>MNVSIEEFTHFDFQLVPEPSPLDLVITESLKNHIEVNGVKSGALLPLPFQTGIGKTYTALNFLLQQMLEQVRSELKEENTGKKSKRLLYYVTDSVDNVVSAKADLLKLIEKQTVKGEPRFTLEQQEYLKAQIVHLPNQSEQLLQCSDAVLNDVLIGFNLNAERDVQAEWSAISGLRRHASNPEVKISLNRQAGYFYRNLIDRLQKKQKGADRVLLSGSLLASVETLLPGEKIRNGSAHVAFLTTSKFLKGFHNTRSRYSPLRDLSGAVLIIDEIDKQNQVILSELCKQQAQDLIWAIRTLRANFRDHQLESSPRYDKIEDLFEPLRERLEEFGTNWNLAFAFNTEGANLNERPVRLFSDRSFTHVSSATHKLSLKSDFLRRKNLIFSDEKVEGSLIEKHGLLTRFVNEADVIYQWFLGTMRKAVFQYWENVRGLEIEVRENRSLEGTFQEAVQSLLTHFNLQEFESAVYESFDTRGLRQSAGGKANKLSSSKSYHHTGLKLVEVAHNQGTRDTVNCKASFLNTSPSGVLADMVDAGAVILGISATARADTVIHNFDFKYLNERLGNKLLSLSREQKQRVNNYYHSRRNYKDNGVVLTVKYLNSRDAFLDALLEEYKPEARSSHFILNHYLGIAESEQAFVRSWLSKLLASIKAFISSPDNRYMLSLLNRTLDTTRQNINDFIQFCCDKWAKEFNVKTKTFFGVNADWMRLVGYDEISKHLNTELGK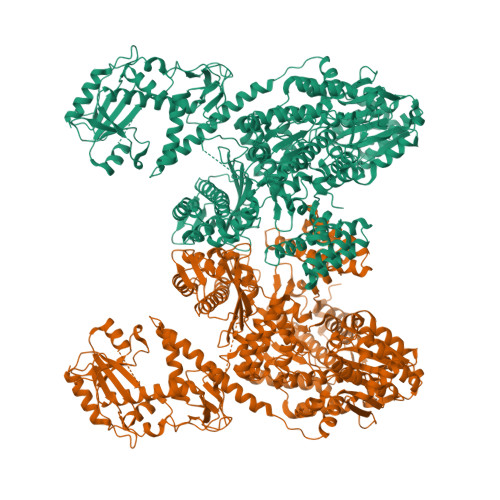VVVFSTYASMGAGKNPDYAVNLALEGESLISVADVTYSTQLRSDIDSIYLEKPTQLLLSDDYSHTANQLCQFHQILSLQENGELSPKSAENWCRQQLMGMSRERSLQQYHQTSDYQSAVRKYIEQAVGRAGRTSLKRKQILLFVDSGLKEILAEESRDPSLFSHEYVALVNKAKSAGKSIVEDRAVRRLFNLAQRNNKDGMLSIKALVHRLHNQPASKSDIQEWQDIRTQLLRYPTVAFQPERFNRLYLQSMTKGYYRYQGNLDGDPNSFEFFDRVPYGDMVSEEDCSLATLVQNQYVRPWFERKGFACSWQKEANVMTPIMFTNIYKGALGEQAVEAVLTAFDFTFEEVPNSIYERFDNRVIFAGIEQPIWLDSKYWKHEGNESSEGYSSKIALVEEEFGPSKFIYVNALGDTSKPIRYLNSCFVETSPQLAKVIEIPALIDDSNADTNRTAVQELIKWLHHS[2x]> AEDWTAALLNRGRSRQPLV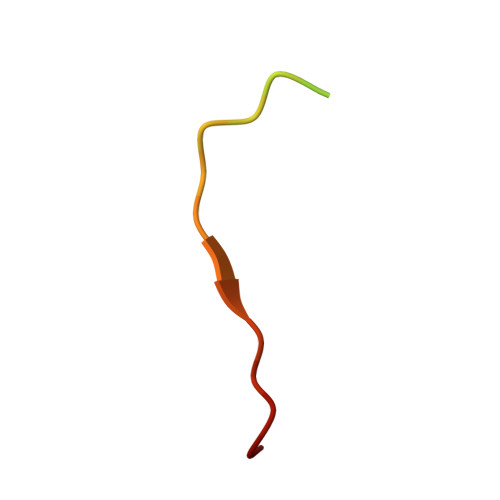LGDNC>[2x]ESSGNKIHFINVQEGGSDAIILESNGHFAMVDTGEDYDFPDGSDSRYPWREGIETSYKHVLTDRVFRRLKELSVQKLDFILVTHTHSDHIGNVDELLSTYPVDRVYLKKYSDSRITNSERLWDNLYGYDKVLQTATETGVSVIQNITQGDAHFQFGDMDIQLYNYENETDSSGELKKIWDDNSNSLIS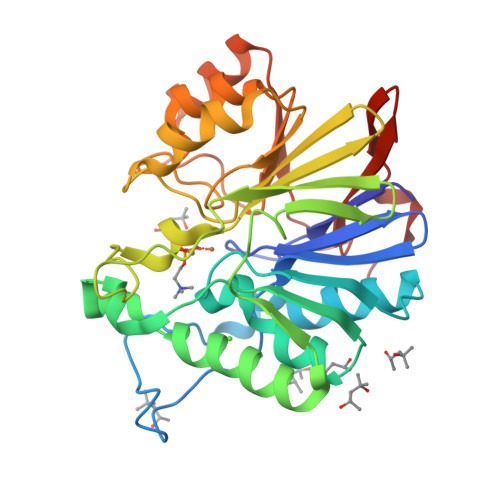VVKVNGKKIYLGGDLDNVHGAEDKYGPLIGKVDLMKFNHHHDTNKSNTKDFIKNLSPSLIVQTSDSLPWKNGVDSEYVNWLKERGIERINAASKDYDATVFDIRKDGFVNISTSYKPIPS> XXXXXXXXXXXXXXXXXXXXXXXXXXXXXXXXXXXXXXXXXXXXXXXXXXXXXXXXXXXXXXXXXXXXXALETVGEKKAFSSVMQLVMTSLQSILENVDTPELLCKCVKCILLVARCYPHIFSTNFRDTVDILVGWHIDHTQKPSLTQQVSGWLQSLEPFWVADLAFSTTLLGQFLEDMEAYAEDLSHVASGESVDEDVPPPSVSLPKLAALLRVFSTVVRSIGERFSPIRGPPITEAYVTDVLYRVMRCVTAANQVFFSEAVLTAANECVGVLLGSLDPSMTIHCDMVITYGLDQLENCQTCGTDYIISVLNLLTLIVEQINTKLPSSFVEKLFIPSSKLLFLRYHKEKEVVAVAHAVYQAVLSLKNIPVLETAYKLILGEMTCALNNLLHSLQLPEACSEIKHEAFKNHVFNVDNAKFVVIFDLSALTTIGNAKNSLIGMWALSPTVFALLSKNLMIVHSDLAVHFPAIQYAVLYTLYSHCTRHDHFISSSLSSSSPSLFDGAVISTVTTATKKHFSIILNLLGILLKKDNLNQDTRKLLMTWALEAAVLMRKSETYAPLFSLPSFHKFCKGLLANTLVEDVNICLQACSSLHALSSSLPDDLLQRCVDVCRVQLVHSGTRIRQAFGKLLKSIPLDVVLSNNKHTEIQEISLALRSHMSKAPSNTFHPQDFSDVISFILYGNSHRTGKDNWLERLFYSCQRLDKRDQSTIPRNLLKTDAVLWQWAIWEAAQFTVLSKLRTPLGRAQDTFQTIEGIIRSLAAHTLNPDQDVSQWTTADNDEGHGNNQLRLVLLLQYLENLEKLMYNAYEGCANALTSPPKVIRTFFYTNRQTCQDWLTRIRLSIMRVGLLAGQPAVTVRHGFDLLTEMKT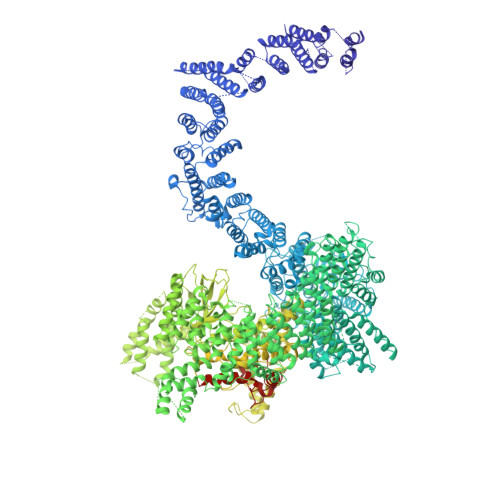TSLSQGNELEVTIMMVVEALCELHCPEAIQGIAVWSSSIVGKNLLWINSVAQQAEGRFEKASVEYQEHLCAMTGVDCCISSFDKSVLTLANAGRNSASPKHSLNGESRKTVLSKPTDSSPEVINYLGNKACECYISIADWAAVQEWQNSIHDLKKSTSSTSLNLKADFNYIKSLSSFESGKFVECTEQLELLPGENINLLAGGSKEKIDMKKLLPNMLSPDPRELQKSIEVQLLRSSVCLATALNPIEQDQKWQSITENVVKYLKQTSRIAIGPLRLSTLTVSQSLPVLSTLQLYCSSALENTVSNRLSTEDCLIPLFSEALRSCKQHDVRPWMQALRYTMYQNQLLEKIKEQTVPIRSHLMELGLTAAKFARKRGNVSLATRLLAQCSEVQLGKTTTAQDLVQHFKKLSTQGQVDEKWGPELDIEKTKLLYTAGQSTHAMEMLSSCAISFCKSVKAEYAVAKSILTLAKWIQAEWKEISGQLKQVYRAQHQQNFTGLSTLSKNILTLIELPSVNTMEEEYPRIESESTVHIGVGEPDFILGQLYHLSSVQAPEVAKSWAALASWAYRWGRKVVDNASXXXXXXXXXXXXXXXXXXXXXXXXXXXXXXXXXXXXXXXXXXEGVIKVWRKVVDRIFSLYKLSCSAYFTFLKLNAGQIPLDEDDPRLHLSHRVEQSTDDMIVMATLRLLRLLVKHAGELRQYLEHGLETTPTAPWRGIIPQLFSRLNHPEVYVRQSICNLLCRVAQDSPHLILYPAIVGTISLSSESQASGNKFSTAIPTLLGNIQGEELLVSECEGGSPPASQDSNKDEPKSGLNEDQAMMQDCYSKIVDKLSSANPTMVLQVQMLVAELRRVTVLWDELWLGVLLQQHMYVLRRIQQLEDEVKRVQNNNTLRKEEKIAIMREKHTALMKPIVFALEHVRSITAAPAETPHEKWFQDNYGDAIENALEKLKXXXXXXXXXXXXXXXXYILRLEEISPWLAAMTNTEIALPGEVSARDTVTIHSVGGTITILPTKTKPKKLLFLGSDGKSYPYLFKGLEDLHLDERIMQFLSIVNTMFATINRQETPRFHARHYSVTPLGTRSGLIQWVDGATPLFGLYKRWQQREAALQAQKAQDSYQTPQNPGIVPRPSELYYSKIGPALKTVGLSLDVSRRDWPLHVMKAVLEELMEATPPNLLAKELWSSCTTPDEWWRVTQSYARSTAVMSMVGYIIGLGDRHLDNVLIDMTTGEVVHIDYNVCFEKGKSLRVPEKVPFRMTQNIETALGVTGVEGVFRLSCEQVLHIMRRGRETLLTLLEAFVYDPLVDWTAGGEAGFAGAVYGGGGQQAESKQSKREMEREITRSLFSSRVAEIKVNWFKNRDEMLVVLPKLDGSLDEYLSLQEQLTDVEKLQGKLLEEIEFLEGAEGVDHPSHTLQHRYSEHTQLQTQQRAVQEAIQVKLNEFEQWITHYQAAFNNLEATQLASLLQEISTQMDLGPPSYVPATAFLQNAGQAHLISQCEQLEGEVGALLQQRRSVLRGCLEQLHHYATVALQYPKAIFQKHRIEQWKTWMEELICNTTVERCQELYRKYEMQYAPQPPPTVCQFITATEMTLQRYAADINSRLIRQVERLKQEAVTVPVCEDQLKEIERCIKVFLHENGEEGSLSLASVIISALCTLTRRNLMMEGAASSAGEQLVDLTSRDGAWFLEELCSMSGNVTCLVQLLKQCHLVPQDLDIPNPMEASETVHLANGVYTSLQELNSNFRQIIFPEALRCLMKGEYTLESMLHELDGLIEQTTDGVPLQTLVESLQAYLRNAAMGLEEETHAHYIDVARLLHAQYGELIQPRNGSVDETPKMSAGQMLLVAFDGMFAQVETAFSLLVEKLNKMEIPIAWRKIDIIREARSTQVNFFDDDNHRQVLEEIFFLKRLQTIKEFFRLCGTFSKTLSGSSSLEDQNTVNGPVQIVNVKTLFRNSCFSEDQMAKPIKAFTADFVRQLLIGLPNQALGLTLCSFISALGVDIIAQVEAKDFGAESKVSVDDLCKKAVEHNIQIGKFSQLVMNRATVLASSYDTAWKKHDLVRRLETSISSCKTSLQRVQLHIAMFQWQHEDLLINRPQAMSVTPPPRSAILTSMKKKLHTLSQIETSIATVQEKLAALESSIEQRLKWAGGANPALAPVLQDFEATIAERRNLVLKESQRASQVTFLCSNIIHFESLRTRTAEALNLDAALFELIKRCQQMCSFASQFNSSVSELELRLLQRVDTGLEHPIGSSEWLLSAHKQLTQDMSTQRAIQTEKEQQIETVCETIQNLVDNIKTVLTGHNRQLGDVKHLLKAMAKDEEAALADGEDVPYENSVRQFLGEYKSWQDNIQTVLFTLVQAMGQVRSQEHVEMLQEITPTLKELKTQSQSIYNNLVSFASPLVTDATNECSSPTSSATYQPSFAAAVRSNTGQKTQPDVMSQNARKLIQKNLATSADTPPSTVPGTGKSVACSPKKAVRDPKTGKAVQERNSYAVSVWKRVKAKLEGRDVDPNRRMSVAEQVDYVIKEATNLDNLAQLYEGWTAWV> MSSAFSGLKIPELSVDPAEVFKSDNPQLVSVLLDEFELQEQRPFFSGLIPEKQINIALKKSPQLKKLACHLLEAYEINGRRWKHADRRRVLEKAIRLLEKVSNELKGDIQKLENNVKESGKDSEELNKTREKHGEILADMGRAYLHRAKIIRPKGFTIPAKKKESLRKALDFCKEAKARHLAGLVGLEMDRCDMSDFDSENSLEKLLRDATTGVSLSKDQYYSNEYRKAEYYQMCIRLAEIEEDKHGATDEGSENNRYKRLEGILGPKKSQGKKKGKKNKKKKGTNSKSALEKIMAFEKFKVAVYLGEGKEKTHWNDFSEFLMRYPFSHPSWEDSVRFLRRLYKKGNDKWRELSVALWEIAKKNSAKTSSIHLRWYWSRQRDLYDLAFLSALEQADIAEDESVRQEKLRLAAKVADSAKNRPALTWQAMEQMADKDEALKKEIENYAQALGGGYIEQFEKTELPKNTNPQDDIPDDLKTSGLVVQFYLVHLKDY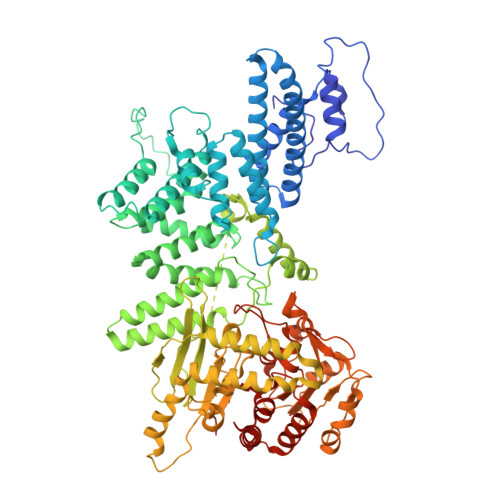ENGYALIYDGKTKKWSCEMFNFFPIWEKYLQWQSVYFDLPANQKEESADQLKALCLELGRHLYFLFDFEENRKAHEKNQDTAKENWDMLFIPHDFLHRVPIHGAIKKNGTNILLKKFNCTYFPTLPNASITPESPKSDNVAELIEYFSEHEKDYSEYFDKIEHIFDKKNRAATSQDLLDAAISPPRTLTIYCHGQSDVNNPFYSRLLLKDKLELIKLATLQEHYSGTHIFLGACETDLMPPLSAPLDEQLSMAAMFLQKGVGSVLGTLWEAYPRAVKDIVKNILSADDTQYFEKLFSLKKKISVNQKKSLYYYLCFKLYRSFDQIGKE> GAACGACACAGA;> CGGTGACTC;> TCTCCG;> TCGAGTCAGTGTCGT

In this work, we exhaustively probe the ability of all 36 immobile HJ sequences to form DNA crystals in two different designed systems. Three separate self-assembling DNA crystal systems are described in this report: the “4 × 5” and “4 × 6” designs (collectively referred to as the 4 × N systems), and a third construct with a “scrambled” sequence variant of the 4 × 6 lattices. Self-assembly was mediated by three constituent oligonucleotides: (S1) containing four sequence repeats of either 5 or 6 bases; (S2) composed of 21 bases containing complementary regions to both (S1); and (S3) which forms the second junction crossover. The HJ serves as the fundamental component at the core of each unit, and the ultimate assembly of the full lattice is facilitated by the complementary 2-base sticky ends that tail each duplex.

To investigate this possibility, we designed “scrambled” sequences with targeted base substitutions, while maintaining GC content, along each “stem”. Contrary to the buffer preference observed with the native P32 crystals, the scrambled systems exhibited an exclusive preference towards low salt buffers, much like the native R3 crystals. Remarkably, only J1 and J2 retained the P32 symmetry, with all others yielding an R3 lattice. The most significant difference between the individual junctions observed in MD simulations was their ability to form distinct potassium ion binding sites near the junction branching point. The mean incidence of binding in the non-fatal junctions was 0.53 (σ = 0.28), suggesting that the ability to capture ions is pivotal to the ability to crystallize the immobile HJs.2-({1-[(4-bromonaphthalen-1-yl)methyl]-1H-imidazo[4,5-b]pyridin-2-yl}sulfanyl)-2-methylpropanoic 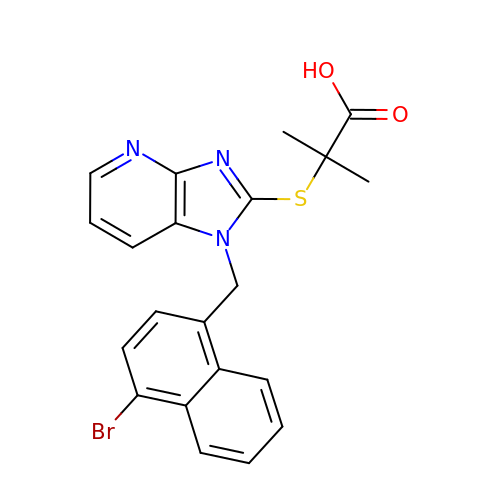acid | C21 H18 Br N3 O2 S | VKHXJKYGFGXZSS-UHFFFAOYSA-N> GPLG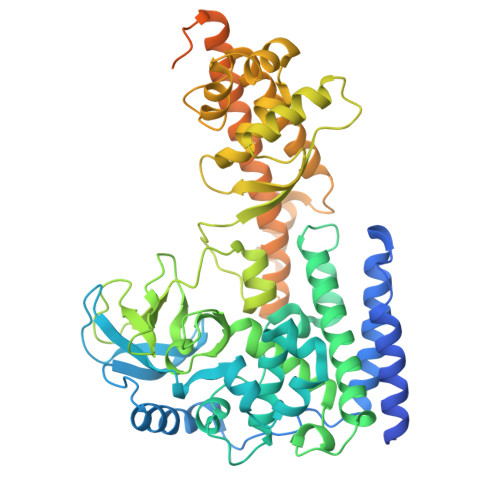SMGKKSRVKTQKSGTGATATVSPKEILNLTSELLQKCSSPAPGPGKEWEEYVQIRTLVEKIRKKQKGLSVTFDGKREDYFPDLMKWASENGASVEGFEMVNFKEEGFGLRATRDIKAEELFLWVPRKLLMTVESAKNSVLGPLYSQDRILQAMGNIALAFHLLCERASPNSFWQPYIQTLPSEYDTPLYFEEDEVRYLQSTQAIHDVFSQYKNTARQYAYFYKVIQTHPHANKLPLKDSFTYEDYRWAVSSVMTRQNQIPTEDGSRVTLALIPLWDMCNHTNGLITTGYNLEDDRCECVALQDFRAGEQIYIFYGTRSNAEFVIHSGFFFDNNSHDRVKIKLGVSKSDRLYAMKAEVLARAGIPTSSVFALHFTEPPISAQLLAFLRVFCMTEEELKEHLLGDSAIDRIFTLGNSEFPVSWDNEVKLWTFLEDRASLLLKTYKTTIEEDKSVLKNHDLSVRAKMAIKLRLGEKEILEKAVKSAAVNREYYRQQMEEKAPLPKYEESNLGLLESSVGDSRLPLVLRNLEEEAGVQDALNIREAISKAKATENGLVNGENSIPNGTRSENESLNQESKRAVEDAKGSSSDSTAGVKE> MKKQDHAHIRTRKARNKELWDSLADFLKGYLVPNLDDNDESIDSLTNEVMLLMKRLIEHDLNLTLNDFSSKTIPIYRLLLRANIITVIEGSTN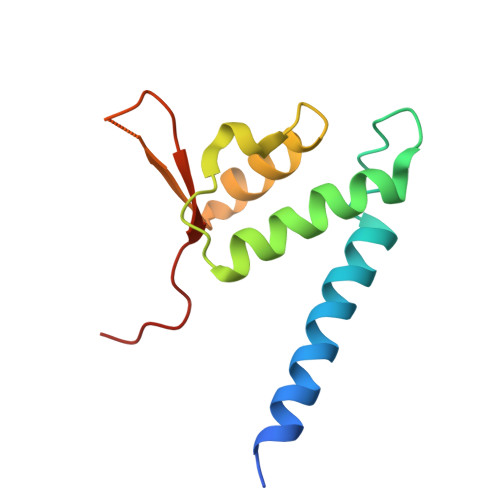PGTKYIKLIDFNETSLT>GIDPFTMASGSAGKPTGEAASPAPASAIGGASSQPRKRLVSVCDHCKGKMQLVADLLLLSSEARPVLFEGPASSGAGAESFEQCRDTIIARTKGLSILTHDVQSQLNMGRFGEAGDSLVELGDLVVSLTECSAHAAYLAAVATPGAQPAQPGLVDRYRVTRCRHEVEQGCAVLRATPLADMTPQLLLEVSQGLSRNLKFLTDACALASDKSRDRFSREQFKLGVKCMSTSASALLACVREVKVAPSELARSRCALFSGPLVQAVSALVGFATEPQFLGRAAAVSAEGKAVQTAILGGAMSVVSACVLLTQCLRDLAQHPDGGAKMSDHRERLRNSACAVSEGCTLLSQALRERSSPRTLPPVNSNSVN[2x]

Talin rod domain–containing protein 1 (TLNRD1) shares 22% homology with the talin R7R8 rod domains, and is highly conserved throughout vertebrate evolution, although little is known about its function. Here we show that TLNRD1 is an α-helical protein structurally homologous to talin R7R8. Like talin R7R8, TLNRD1 binds F-actin, but because it forms a novel antiparallel dimer, it also bundles F-actin. Increasing TLNRD1 expression enhances filopodia formation and cell migration on 2D substrates, while TLNRD1 down-regulation has the opposite effect. Together, our results suggest that TLNRD1 has retained the diverse interactions of talin R7R8, but has developed distinct functionality as an actin-bundling protein that promotes filopodia assembly.

To determine the extent of the structural similarity between TLNRD1 and talin R7R8, we used x-ray crystallography to solve the structures of both full-length TLNRD1 (TLNRD1-FL) and the four-helix domain (TLNRD1-4H). This confirmed that TLNRD1 consists of a nine-helix module comprised of a four-helix and five-helix bundle connected via the same unusual domain linkage identified in talin R7R8, where the four-helix bundle (R8) is inserted into a loop between helices α3 and α4 of the five-helix bundle (R7). The first 40 residues of TLNRD1-FL are not visible in the density, supporting the secondary structure prediction that the N-terminal region is unstructured. The TLNRD1 structures reveal the basis for TLNRD1 dimerization, which is mediated by a novel interface on the four-helix bundle. In both the TLNRD1-FL and TLNRD1-4H structures, the four-helix bundle forms an extensive interaction with a four-helix bundle of a second TLNRD1 molecule. An identical dimer interface was observed in both the TLNRD1-FL and the TLNRD1-4H structures, which crystallized in different space groups. However, the structure of TLNRD1 revealed that the putative actin-binding surfaces on α2 and α3 are positioned facing away from the dimer interface, raising the possibility that TLNRD1 might engage two actin filaments simultaneously, and thus cross-link and bundle actin. However, a notable feature of the TLNRD1-FL structure is that the five-helix bundle packs against the side of the four-helix bundle. Thus, it is possible that this more compact conformation might represent an autoinhibited conformation of TLNRD1, rendering some binding sites cryptic. The structural information from equivalent talin complexes was used to model the RIAM- and KANK-binding sites onto the TLNRD1-FL structure.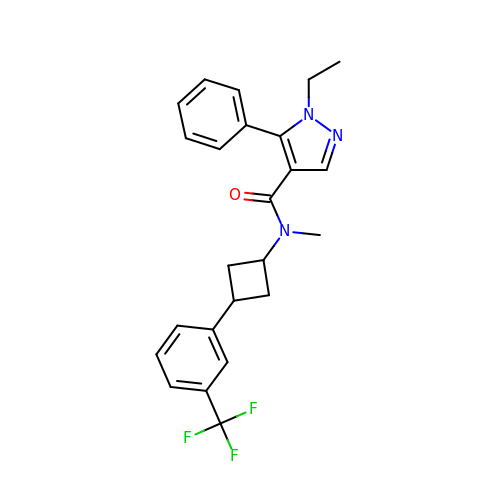1-ethyl-~{N}-methyl-5-phenyl-~{N}-[3-[3-(trifluoromethyl)phenyl]cyclobutyl]pyrazole-4-carboxamide | C24 H24 F3 N3 O | VWSNDEZRLZHMNM-PUZFROQSSA-N(1S)-2-[(2S)-2-methyl-3-sulfanyl-propanoyl]-3,4-dihydro-1H-isoquinoline-1-carboxylic acid | C14 H17 N O3 S | 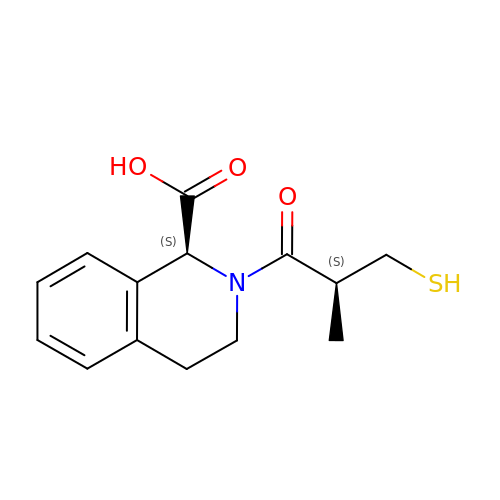DMGKNMLYAQKRNE-SKDRFNHKSA-N> MTEK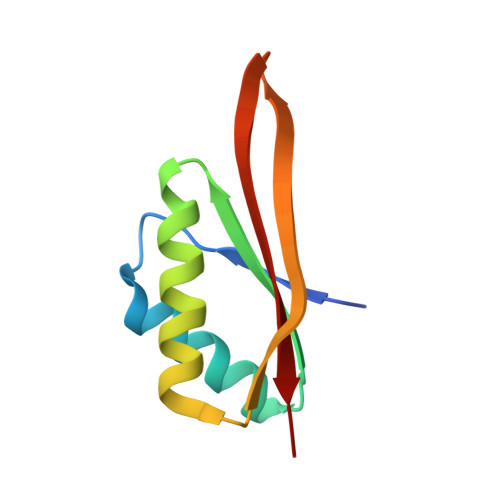LNEIVVRKTKNVEDHVLDVIVLFNQGIDEVILKGTGREISKAVDVYNSLKDRLGDGVQLVNVQTGSEVRDRRRISYILLRLKRVY> GC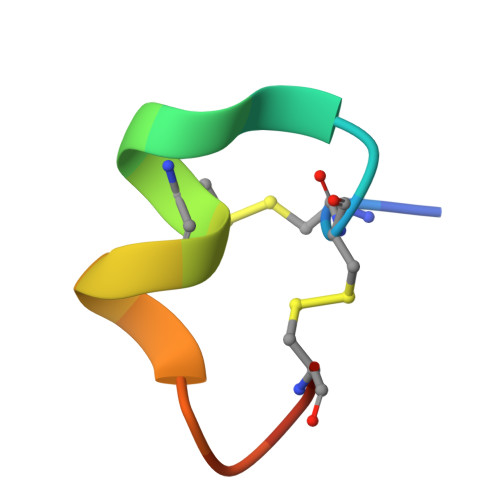CSHPACNVAHPEICX>[8x]GSHMSASAELEPDVKGRILDAAADAFMA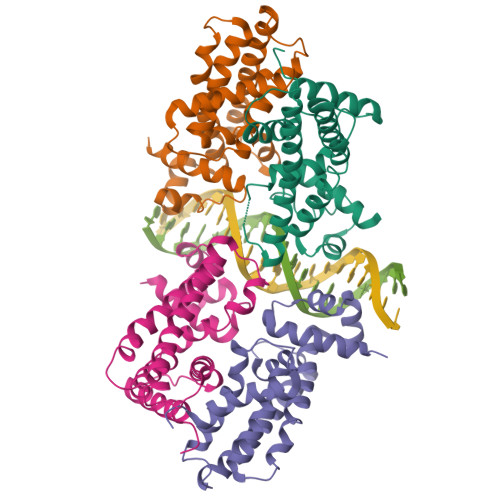RGFANTTIDDIADEVGATKGLIYYHFRSKFDIFLAVYEDGMRRVRERVEPHSTAPGTGHQRLEAMSIAHLENLMTELGYHHVVHQGVRHQDSTALKVRQRDALTALNELRRDYERMFRRVIAEGIADGSLRRVDEALATRTLLSNLNAVDVWYRKIEGQTGEEIRELASQVVDMLIGGLAD>GSGMSYTMCSGKFSIDKEMAETQHGTTVVKVKYEGAGAPCKVPIEIRDVNKEKVVGRIISSTPLAENTNSVT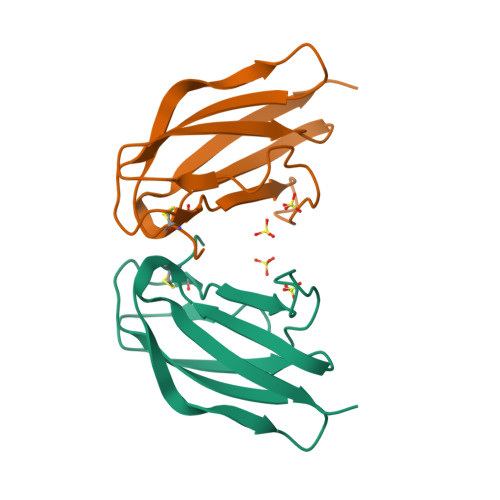NIELEPPFGDSYIVIGVGNSALTIHWFRKGSSIGK[3x]>MAENTKNENITNILTQKLIDTRTVLIYGEINQELAEDVSKQLLLLESISNDPITIFINSQGGHVEAGDTIHDMIKFIKPTVKVVGTGWVASAGITIYL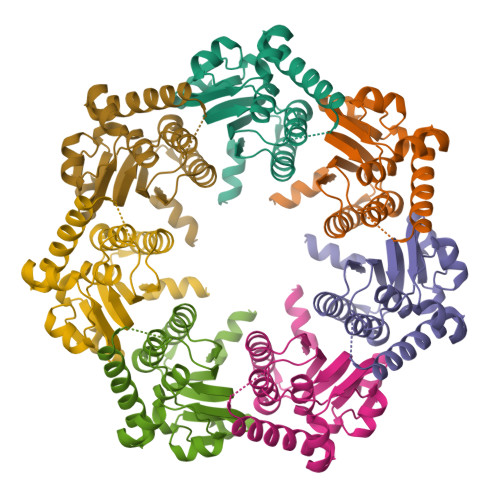AAEKENRFSLPNTRYMIHQPAGGVQGQSTEIEIEAKEIIRMRERINRLIAEATGQSYEQISKDTDRNFWLSVNEAKDYGIVNEIIENRDGLKMASWSHPQFEK[28x]>MPNYKLTYFNMRGRAEIIRYIFAYLDIQYEDHRIEQADWPEIKSTLPFGKIPILEVDGLTLHQSLAIARYLTKNTDLAGNTEMEQCHVDAIVDTLDDFMSCFPWAEKKQDVKEQMFNELLTYNAPHLMQDLDTYLGGREWLIGNSVTWADFYWEICSTTLLVFKPDLLDNHPRLVTLRKKVQAIPAVA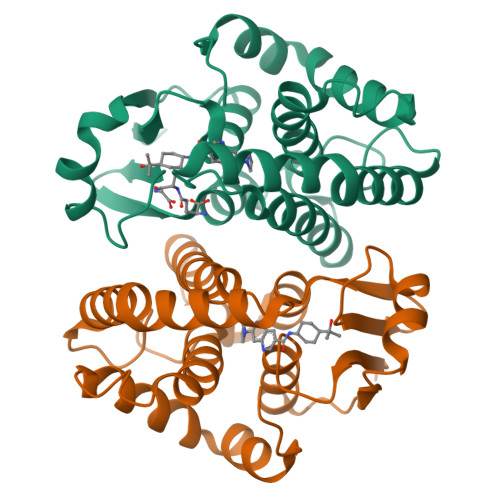NWIKRRPQTKL[2x]> SEFGHRTLASTPALWASIPCPRSELRLDLVLPSGQSFRWREQSPAHWSGVLADQVWTLTQTEEQLHCTVYRGDKSQASRPTPDELEAVRKYFQLDVTLAQLYHHWGSVDS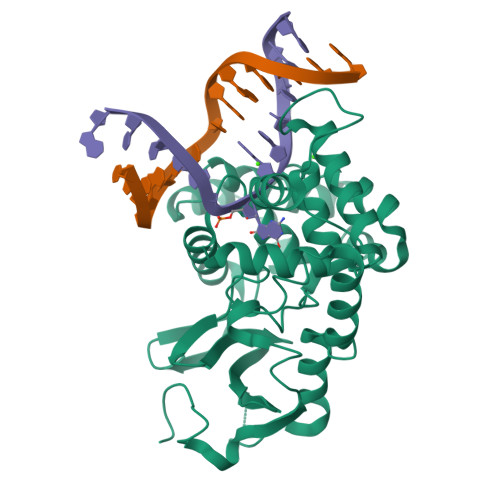HFQEVAQKFQGVRLLRQDPIECLFSFICSSCNNIARITGMVERLCQAFGPRLIQLDDVTYHGFPSLQALAGPEVEAHLRKLGLGYRARYVSASARAILEEQGGLAWLQQLRESSYEEAHKALCILPGVGTKVADCICLMALDKPQAVPVDVHMWHIAQRDYSWHPTTSQAKGPSPQTNKELGNFFRSLWGPYAGWAQAVLFSADLRQ> MRIDPFKLAHWMNARKYTAAQTADLAGLPLDDLRRLLGDEANEPDPAAATALAEALSVEPSQLAADAHRNLTVVHKSAEEMHASRRPIQRDGIHFYNYYTLAAPEGRVAPVVLDILCPSDRLPALNNGHLEPAITVNLGPGDINGRWGEEITPQTWRVLHANHGGDRWITGDSYVHPSYCPHSYSL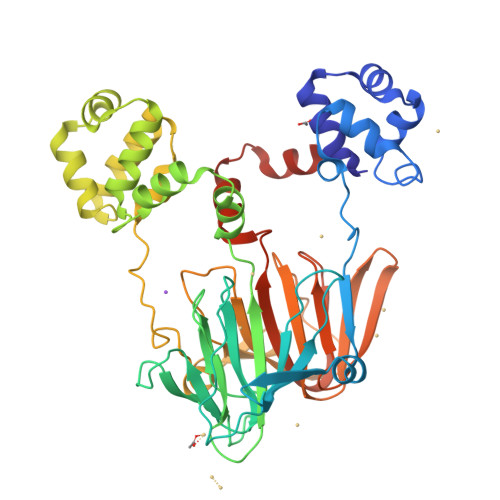AGDAPARIVSYTAQSNISPLMTEANNWSTGAFEEALKALSGKVSAGSVLDLFLARRAHTRTSAAEAAGVPPADLEAALRSPASETGLTVLRTLGRALGFDYRVLLPADDQHDGVGKTWTTIEDSRRSRRTFGTYEAASMASAAHLPDLVGSFLRVDADGRGADLIDHAENHYVVTEGRLTLEWDGPDGPASVELEPDGSAWTGPFVRHRWHGTGTVLKFGSGAHLGYQDWLELTNTFEPAATLRRGRRDLAGWGYDN> VRWARALYDFEALEEDELGFRSGEVVEVLDSSNPSWWTGRLHNKLGLFPANYVA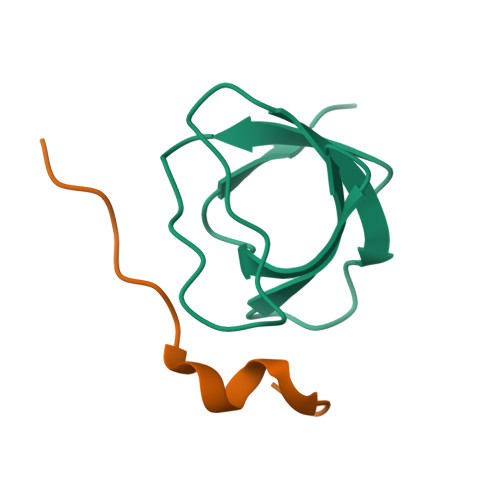PMMR;> GQPPLVPPRKEKMRGK> 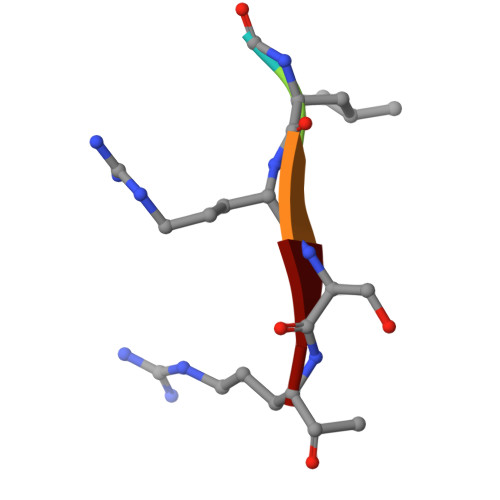ALRSX> MRVLLIHADYFEYEVKDKALKNPEPISEDMKRGRMEEVLVAWISVEKVDEKNPEEVSLKAIEEISKVAEQVKAENVFVAPWAHLSSELAKPSVAMDILNRVYQGLKE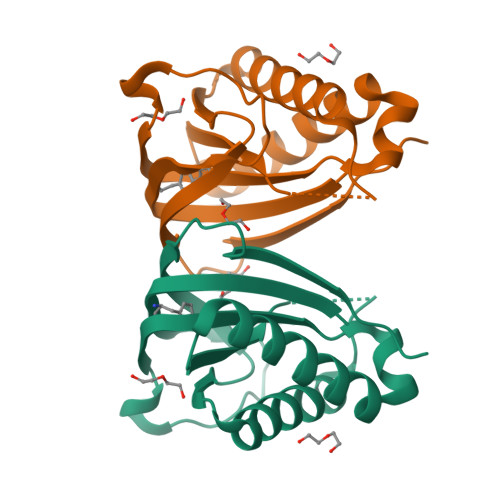RGFNVGKAPFGYYIAYKISCKGHPLAELSRTIVPEELEHHHHHH The glucose-dependent respiration of bloodstream forms of the parasite Trypanosoma brucei depends on an unusual and essential mitochondrial electron-transport system, consisting of glycerol-3-phosphate dehydrogenase and the trypanosome alternative oxidase (TAO). Clarkson et al. first demonstrated that the respiratory pathway of the T. brucei bloodstream trypomastigotes is solely dependent on a “plant-like alternative oxidase” now known as the trypanosome alternative oxidase (TAO), which is located in the inner mitochondrial membrane of the parasite. The active site of TAO is mapped by the presence of di-iron and a hydroxo ion. The cavity has been described to be a ubiquinol substrate binding site and the oxygen trough.

We compared the structure of both forms of the enzyme and found the structural conformations to be largely the same all over the molecule, except at the active site. Figure A shows the active site in the ligand-free form to be in an open conformation, while upon binding of compound 1, the active site of TAO assumes a closed conformation. The cavity was open when 1 was not bound.

>[4x]TPVWGHTQLNRLSFLETVPVVPLRVSDESSEDRPTWSLPDIENVAITHKKPNGLVDTLAYRSVRTCRWLFDTFSLYRFGSITESKVISRCLFLETVAGVPGMVGGMLRHLSSLRYMTRDKGWINTLLVEAENERMHLMTFIELRQPGLPLRVSIIITQAIMYLFLLVAYVISPRFVHRFVGYLEEEAVITYTGVMRAIDEGRLRPTKNDVPEVARVYWNLSKNATFRDLINVIRADEAEHRVVNHTFADMHEKRLQNSVNPFVVLKKNPEE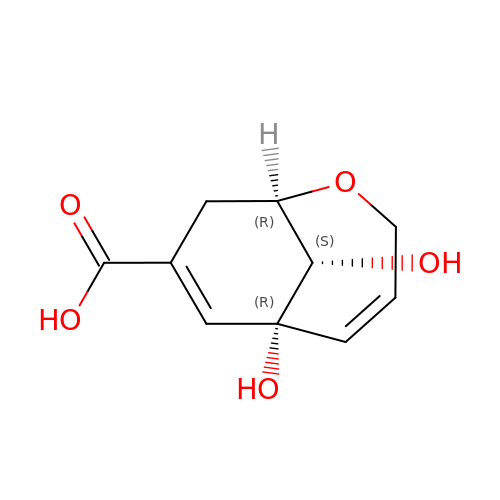(1R,6R,10S)-6,10-dihydroxy-2-oxabicyclo[4.3.1]deca-4(Z),7-diene-8-carboxylic acid | C10 H12 O5 | RGHXALVTPJSFBL-KHQFGBGNSA-N Our comparative bioinformatics studies suggest that among those reported as glycosyltransferases are also pseudo-glycosyltransferases (such as VldE, EC 2.x.x.x), which do not recognize sugars as substrates but rather catalyze the formation of non-glycosidic C-N bonds in the biosynthesis of C7N-aminocyclitol-containing natural products such as acarbose and validamycin A. Validoxylamine A is generated through the dephosphorylation of validoxylamine A 7′-phosphate by VldH while validoxylamine A 7′-phosphate (VDO) results from a condensation of GDP-valienol and validamine 7-phosphate (both are pseudo-sugars) by the pseudo-glycosyltransferase, VldE. Similar to OtsA, VldE is comprised of two Rossman β/α/β domains which are oriented in a GT-B configuration. As was described in a recent crystallographic study of ValL, a VldE homolog from S. hygroscopicus subsp. jinganggensis, VldE is a homodimer.

The GDP bound structure of VldE (VldE•GDP) described here is also in an “open” conformation and the binding of GDP did not have an effect on the global conformation of the apo enzyme (RMSD Cα = 0.350 Å). Within VldE, the ribose and phosphate moieties of GDP make interactions with the side-chains of the residues Arg290, Lys 295 and Glu391; as well as with the backbone atoms of residues Leu387 and Ser388. The α-phosphate of GDP does make a single unique interaction with Ser388 within VldE. This interaction is not possible within OtsA as there is a valine at the same position. Nonetheless, the ribose and phosphate moieties of GDP within the VldE catalytic pocket are nearly superimposable (RMSD = 0.868) onto the ribose and phosphate moieties of UDP within the OtsA catalytic pocket. The guanine moiety within the VldE•GDP complex makes interactions with the hydrophilic residues Arg321, Asn323, and Thr366. The preference of guanine by VldE is mediated by these three hydrophilic residues, while the preference for a uracil moiety is mediated by three hydrophobic residues at the same positions. Within OtsA, the uracil is surrounded by the hydrophobic residues Ile295, Pro297, and Leu344. The preference of a GDP activated donor sugar by VldE (instead of UDP) is immediately apparent when comparing the catalytic site to that of OtsA. The conserved position of the β-phosphate of GDP is critically important because the bond between this phosphate and the donated cyclitol is broken during the transfer to the acceptor.

>MTGSEIFLASKRAAITYDTDPATGEPRAWLAPGGTGNVVAEQAGVLNISWIASADSEDDRRASALNPDGVTMELHSGREILVRLIRHDPAVFRNVQNFMTANLMWAANNYGWDRWTQPSFGSDAREGWADFGRFTRDFADAILKSSAQSADPVYLVHDYQLVGVPALLREQRPDAPILLFVHIPWPSADYWRILPKEIRTGILHGMLPATTIGFFADRWCRNFLESVADLLPDARIDREAMTVEWRGHRTRLRTMPLGYSPLTLDGRNPQLPEGIEEWADGHRLVVHSGRTDPIKNAERAVRAFVLAARGGGLEKTRMLVRMNPNRLYVPANADYVHRVETAVAEANAELGSDTVRIDNDNDVNHTIACFRRADLLIFNSTVDGQNLSTFEAPLVNERDADVILSETCGAAEVLGEYCRSVNPFDLVEQAEAISAALAAGPRQRAEAAARRRDAARPWTLEAWVQAQLDGLAADHAARTATAERFDTAPAVSTRADL[2x]>RVVCREASHAGSWYTASGPQLNAQLEGWLSQVQSTKRPARAIIAPHAGYTYCGSC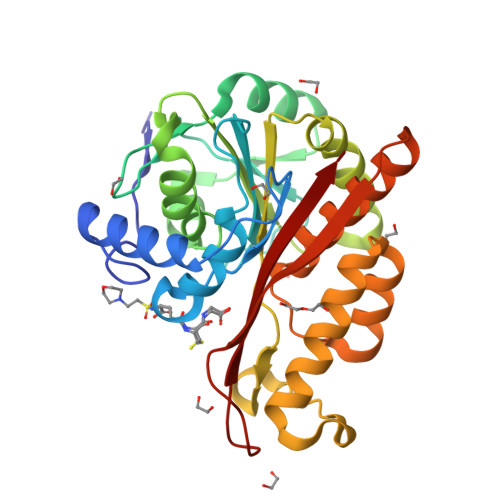AAHAYKQVDPSITRRIFILGPSHHVPLSRCALSSVDIYRTPLYDLRIDQKIYGELWKTGMFERMSLQTDEDEHSIEMHLPYTAKAMESHKDEFTIIPVLVGALSESKEQEFGKLFSKYLADPSNLFVVSSDFCHWGQRFRYSYYDESQGEIYRSIEHLDKMGMSIIEQLDPVSFSNYLKKYHNTISGRHPIGVLLNAITELQKNGMNMSFSFLNYAQSSQCRNWQDSSVSYAAGALTVH[4x]>[5x]MFSGIKGPNPSDLKGPELRILIVHARWNLQAIEPLVKGAVETMIEKHDVKLENIDIESV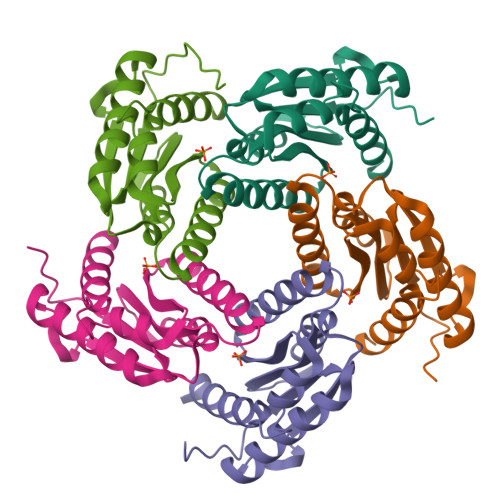PGSYELPQGIRASIARNTYDAVIGIGVLIKGSTMHFEYISEAVVHGLMRVGLDSGVPVILGLLTVLNEEQALYRAGLNGGHNHGNDWGSAAVEMGLKALY>MTDTTLPPDDSLDRIEPVDIEQEMQRSYIDYAMSVIVGRALPEVRDGLKPVHRRVLYAMFDSGFRPDRSHAKSARSVAETMGNYHPHGDASIYDSLVRMAQPWSLRYPLVDGQGNFGSPGNDPPAAMRYTEARLTPLAMEMLREIDEETVDFIPNYDGRVQEPTVLPSRF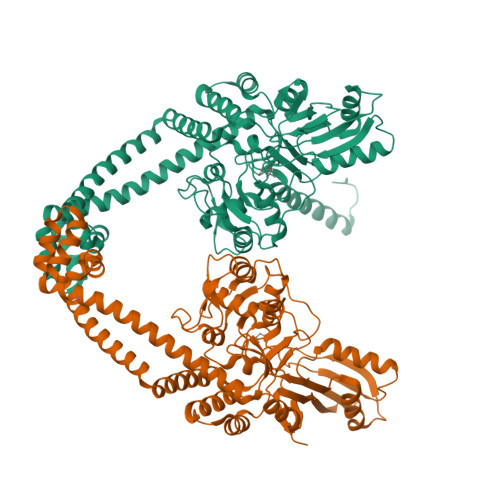PNLLANGSGGIAVGMATNIPPHNLRELADAVFWALENHDADEEETLAAVMGRVKGPDFPTAGLIVGSQGTADAYKTGRGSIRMRGVVEVEEDSRGRTSLVITELPYQVNHDNFITSIAEQVRDGKLAGISNIEDQSSDRVGLRIVIEIKRDAVAKVVINNLYKHTQLQTSFGANMLAIVDGVPRTLRLDQLIRYYVDHQLDVIVRRTTYRLRKANERAHILRGLVKALDALDEVIALIRASETVDIARAGLIELLDIDEIQAQAILDMQLRRLAALERQRIIDDLAKIEAEIADLEDILAKPERQRGIVRDELAEIVDRHGDDRRTRIIAAEHHHHHH[2x]> XIWIAQELRSRGDSFN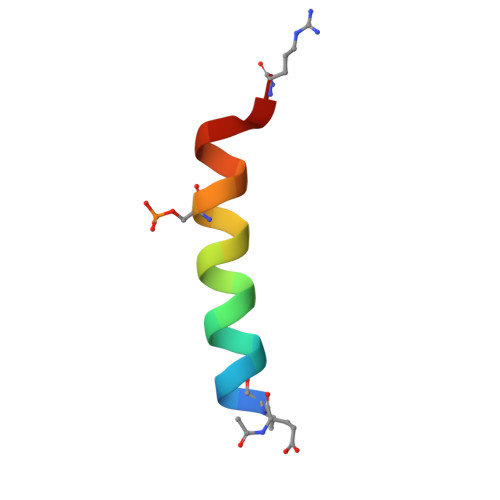AYYAR> MKSVAILAALFGSATAFVPSQVSRTAASTSVKASLADMVGAEGPEPIPFAPSKTSKNFDPVGFAERSPEWLPWYREAELKHGRA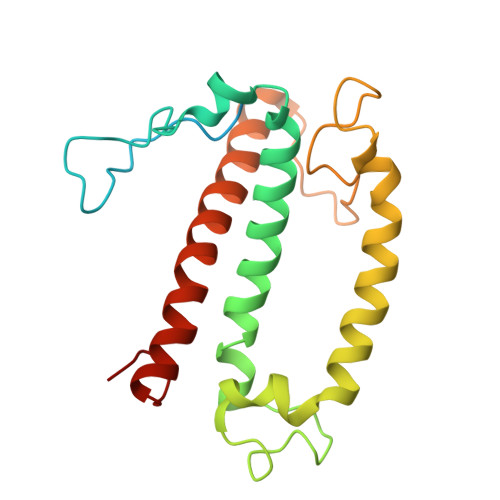AMLATVGFVVPEFIRVPGEQFSFEAIPKVIDAHDALPESMIQIFGWISFLEACTFPAMAGLGGKYDRKPGDFSFDPLGLYPTDPEKQKQMQLAELKNGRLAMIAIGGMVTGAAVTGHGFPYLP> ETGNKYIEKRAIDLSRERDPNFFDNPGIPVPECFWFMFKNNVRQDAGTCYSSWKMDMKV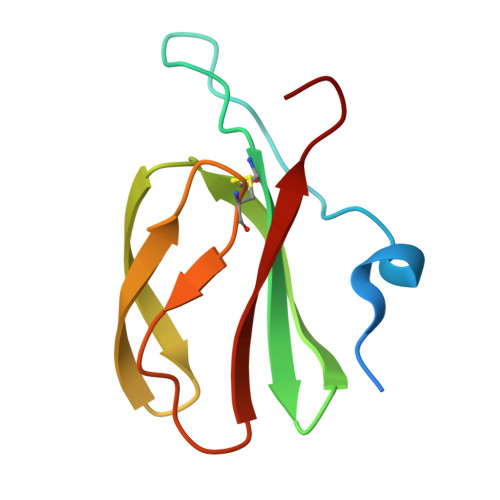GPNWVHIKSDDNCNLSGDFPPGWIVLGKKRPGF> MGWSLPKEKGLILCLWNKFCRWFHRRESWAQSRDEQNLLQQKRIWESPLLLAAKENNVQALYKLLKFEGCEVHQKGAMGETALHIAALYDNNEAAQVLMEAAPELVFEPMTSELYEGQTALHIAVINQNVNLVRALLARGASVSARATGSVFHYRPHNLIYYGEHPLSFAACVGSEEIVRLLIEHGADIRAQDSLGNTVLHILILQPNKTFACQMYNLLLSYDGGDHLKSLELVPNNQGLTPFKLAGVEGNIVMFQHLMQKRKHIQWTYGPLTSTLYDLTEIDSSGDDQSLLELIVTTKKREARQILDQTPVKELVSLKWKRYGRPYFCVLGAIYVLYIICFTMCCVYRPLKPRITNRTNPRDNTLLQQKLLQEAYVTPKDDLRLVGELVSIVGAVIILLVEIPDIFRLGVTRFFGQTILGGPFHVIIVTYAFMVLVTMVMRLTNSDGEVVPMSFALVLGWCNVMYFARGFQMLGPFTIMIQKMIFGDLMRFCWLMAVVILGFASAFYIIFQTEDPDELGHFYDYPMALFSTFELFLTIIDGPANYDVDLPFMYSITYAAFAIIATLLMLNLLIAMMGDTHWRVAHERDELWRAQVVATTVMLERKLP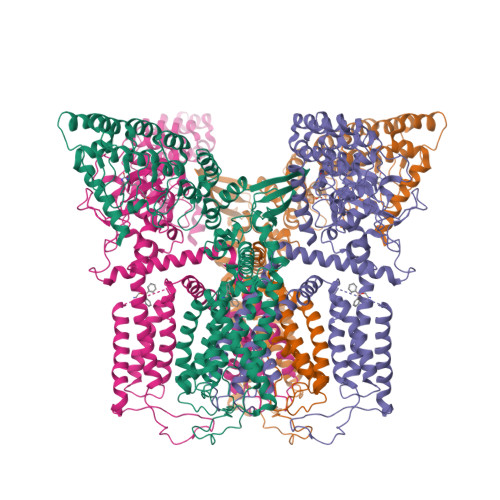RCLWPRSGICGREYGLGDRWFLRVEDRQDLNRQRIRRYAQAFQQQDDLYSEDLEKDSGEKLVPR Glypicans are heparan sulfate proteoglycans that are attached to the cell-membrane surface by glycosylphosphatidylinositol anchorage. Glypican-1 (Gpc-1) is the predominant heparan sulfate proteoglycan in the developing and adult human brain and is involved in regulation of neurogenesis, axon guidance and synaptogenesis. Recently, we determined the crystal structure of N-glycosylated human glypican-1 core protein at 2.55 Å resolution, which revealed a cylindrical all-α-helical fold (dimensions 120 × 30 × 30 Å) decorated with three major loops and containing the 14 cysteine residues that are conserved in all members of the glypican family. A study has been carried out to establish whether controlled dehydration could be used to improve the anisotropy of crystals of the core protein of the human proteoglycan glypican-1.

The best diffraction data set (2.46 Å resolution) was collected from a crystal dehydrated using the script (86%, 0.1%, 30 s) with a total incubation time of 65 min. These data had an anisotropy ΔB of 13.6 Å2 when checked with the UCLA MBI Diffraction Anisotropy Server, while the control data, without dehydration, had a strong anisotropy ΔB of 40.7 Å2. Also, the Wilson B factor was reduced by 25% to 36.8 Å2, which reveals significant improvement in the degree of short-range lattice order in the crystal after dehydration. After dehydration the overall model B factor fell from 73.8 to 61.4 Å2, which is in better agreement with the corresponding values found in 700 structures refined at the same resolution (using phenix.polygon). Shrinkage of the unit cell after dehydration leads to tighter packing, decreasing the flexible areas and forming new lattice contacts, mainly along the c axis. The new density maps allowed the building of more complete models for all of the Gpc-1 monomers in the asymmetric unit and displayed well defined side-chain density, allowing more reliable side-chain placement. In the dehydrated Gpc-1 crystals the orientation with respect to each other of the pairs of chains A/B and C/D is preserved (almost no rotation and <1 Å translation of B relative to A), while the pair C/D undergoes an almost pure translation of about 11 Å relative to A/B. This translation results in the creation of a new intermolecular interface. The trans­lation peak, now at (½, 0.0742, ½), increases to 42% of the height of the origin peak. Together with the reduction in the β angle from 94.6 to 90.8°, this suggests an ongoing transition to face-­centred orthorhombic symmetry, but within the range of parameters investigated here we did not achieve a complete transition.

>[4x]APQLHHHHHHDLYENLYFQGKLDPASKSRSCGEVRQIYGAKGFSLSDVPQAEISGEHLRICPQGYTCCTSEMEENLANRSHAELETALRDSSRVLQAMLATQLRSFDDHFQHLLNDSERTLQATFPGAFGELYTQNARAFRDLYSELRLYYRGANLHLEETLAEFWARLLERLFKQLHPQLLLPDDYLDCLGKQAEALRPFGEAPRELRLRATRAFVAARSFVQGLGVASDVVRKVAQVPLGPECSRAVMKLVYCAHCLGVPGARPCPDYCRNVLKGCLANQADLDAEWRNLLDSMVLITDKFWGTSGVESVIGSVHTWLAEAINALQDNRDTLTAKVIQGCGNPKVNPQGPGPEEKRRRGKLAPRERPPSGTLEKLVSEAKAQLRDVQDFWISLPGTLCSEKMALSTASDDRCWNGMARGRYLPEVMGDGLANQINNPEVEVDITKPDMTIRQQIMQLKIMTNRLRSAYNGNDVDFQ>[2x]MSDPIVHFNGTHEALLNRIKEAPGLVLVDFFATWCGPCQRLGQILPSIAEANK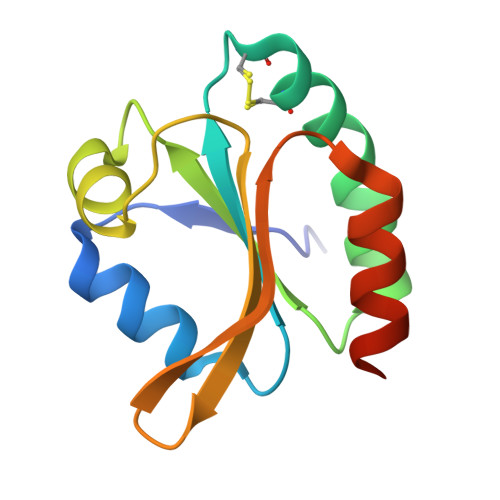DVTFIKVDVDKNGNAADAYGVSSIPALFFVKKEGNEIKTLDQFVGADVSRIKADIEKFKHHHHHH> PLGVQGLTEEQRMMIRELMDAQMKTFDTTFSHFKNFRLPGVLSSGCELPESLQAPSREEAAKWSQVRKDLCSLKVSLQLRGEDGSVWNYKPPADSGGKEIFSLLPHMADMSTYMFKGIISFAKVISYFRDLPIEDQISLLKGAAFELCQLRFNTVFNAETGTWECGRLSYCLEDTAGGFQQLLLEPMLKFHYMLKKLQLHEEEYVLMQAISLFSPDRPGVLQHRVVDQLQEQFAITLKSYIECNRPQPAHRFLFLKIMAMLTELRSINAQHTQRLLRIQDIHPFATPLMQELFG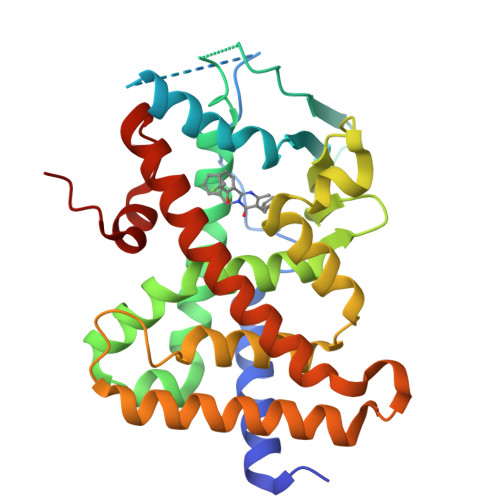ITGS>GMSDPGNEQNGDGIDPAIVEVLLVLREAGIENGATPWSLPKIAKRAQLPMSVLRRVLTQLQAAGLADVSVEADGRGHASLTQEGAAL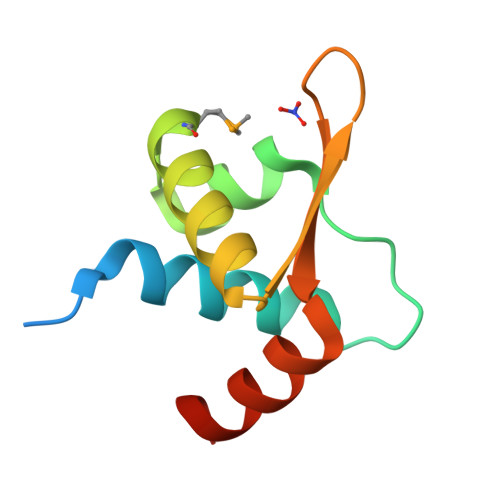AAQLFPDPF[2x]> MSSFIQYEFLKIYQGNQKIKNYYKRKRLIFQQKKVLKKKQKEIQMSTNNLRLKPWFHWTDEERSHAIFSAYEKRILKSEDLPSFLRANRINNVSTWVFPLIALPLFNQSIFKLGFAQRILLTRPAIEWHCFKIATVAASWLAWLNFSPFYRKLENEKEYLLDTLESRIGINVLDLNDALPRWTTSQEYNRRTQQLYNQRNGFFAGLLYPQEESSRP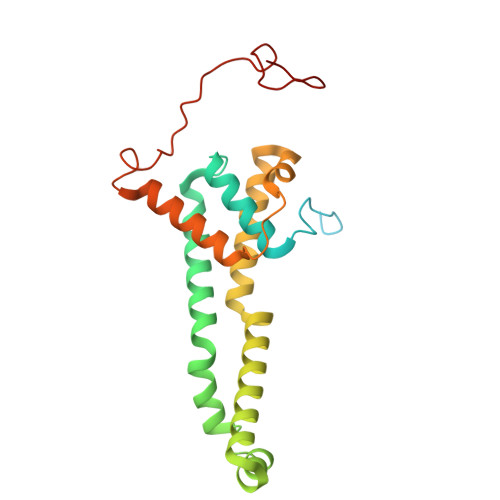LVDIASFPKNLHKEKLTK> MSVFDRLAGFADSVTNAKQVDVSTATAQKKAEQGVTTPLVSPDAAYQMQAARTGNVGANAFEPGTVQSDFMNLTPMQIMNKYGVEQGLQLINARADAGNQVFNDSVTTRTPGEELGDIATGVGLGFVNTLGGIGALGAGLLNDDAGAVVAQQLSKFNDAVHATQSQALQDKRKLFAARNLMNEVESERQYQTDKKEGTNDIVASLSKFGRDFVGSIENAAQTDSIISDGLAEGVGSLLGAGPVLRGASLLGKAVVPANTLRSAALAGAIDAGTGTQSLARIASTVGRAAPGMVGVGAMEAGGAYQQTADEIMKMSLKDLEKSPVYQQHIKDGMSPEQARRQTASETGLTAAAIQLPIAAATGPLVSRFEMAPFRAGSLGAVGMNLARETVEEGVQGATGQLAQNIAQQQNIDKNQDLLKGVGTQAGLGALYGFGSAGVVQAPAGAARLAGAATAPVLRTTMAGVKAAGSVAGKVVSPIKNTLVARGERVMKQNEEASPVADDYVAQAAQEAMAQAPEAEVTIRDAVEATDATPEQKVAAHQYVSDLMNATRFNPENYQEAPEHIRNAVAGSTDQVQVIQKLADLVNTLDESNPQALMEAASYMYDAVSEFEQFINRDPAALDSIPKDSPAIELLNRYTNLTANIQNTPKVIGALNVINRMINESAQNGSLNVTEESSPQEMQNVALAAEVAPEKLNPESVNVVLKHAADGRIKLNNRQIAALQNAAAILKGAREYDAEAARLGLRPQDIVSKQIKTDESRTQEGQYSALQHANRIRSAYNSGNFELASAYLNDFMQFAQHMQNKVGALNEHLVTGNADKNKSVHYQALTADREWVRSRTGLGVNPYDTKSVKFAQQVALEAKTVADIANALASAYPELKVSHIKVTPLDSRLNAPAAEVVKAFRQGNRDVASSQPKADSVNQVKETPVTKQEPVTSTVQTKTPVSESVKTEPTTKESSPQAIKEPVNQSEKQDVNLTNEDNIKQPTESVKETETSTKESTVTEELKEGIDAVYPSLVGTADSKAEGIKNYFKLSFTLPEEQKSRTVGSEAPLKDVAQALSSRARYELFTEKETANPAFNGEVIKRYKELMEHGEGIADILRSRLAKFLNTKDVGKRFAQGTEANRWVGGKLLNIVEQDGDTFKYNEQLLQTAVLAGLQWRLTATSNTAIKDAKDVAAITGIDQALLPEGLVEQFDTGMTLTEAVSSLAQKIESYWGLSRNPNAPLGYTKGIPTAMAAEILAAFVESTDVVENIVDMSEIDPDNKKTIGLYTIT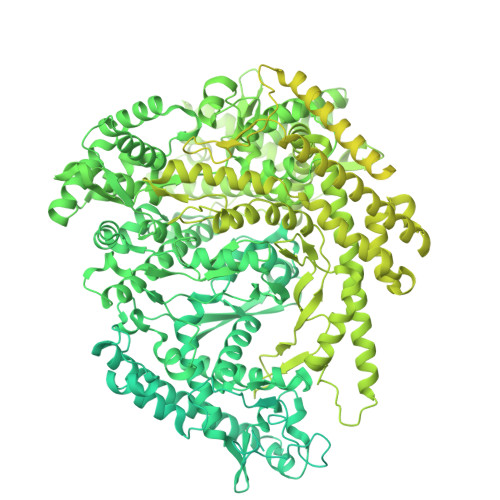ELDSFDPINSFPTAIEEAVLVNPTEKMFFGDDIPPVANTQLRNPAVRNTPEQKAALKAEQATEFYVHTPMVQFYETLGKDRILELMGAGTLNKELLNDNHAKSLEGKNRSVEDSYNQLFSVIEQVRAQSEDISTVPIHYAYNMTRVGRMQMLGKYNPQSAKLVREAILPTKATLDLSNQNNEDFSAFQLGLAQALDIKVHTMTREVMSDELTKLLEGNLKPAIDMMVEFNTTGSLPENAVDVLNTALGDRKSFVALMALMEYSRYLVAEDKSAFVTPLYVEADGVTNGPINAMMLMTGGLFTPDWIRNIAKGGLFIGSPNKTMNEHRSTADNNDLYQASTNALMESLGKLRSNYASNMPIQSQIDSLLSLMDLFLPDINLGENGALELKRGIAKNPLTITIYGSGARGIAGKLVSSVTDAIYERMSDVLKARAKDPNISAAMAMFGKQAASEAHAEELLARFLKDMETLTSTVPVKRKGVLELQSTGTGAKGKINPKTYTIKGEQLKALQENMLHFFVEPLRNGITQTVGESLVYSTEQLQKATQIQSVVLEDMFKQRVQEKLAEKAKDPTWKKGDFLTQKELNDIQASLNNLAPMIETGSQTFYIAGSENAEVANQVLATNLDDRMRVPMSIYAPAQAGVAGIPFMTIGTGDGMMMQTLSTMKGAPKNTLKIFDGMNIGLNDITDASRKANEAVYTSWQGNPIKNVYESYAKFMKNVDFSKLSPEALEAIGKSALEYDQRENATVDDIANAASLIERNLRNIALGVDIRHKVLDKVNLSIDQMAAVGAPYQNNGKIDLSNMTPEQQADELNKLFREELEARKQKVAKARAEVKEETVSEKEPVNPDFGMVGREHKASGVRILSATAIRNLAKISNLPSTQAATLAEIQKSLAAKDYKIIYGTPTQVAEYARQKNVTELTSQEMEEAQAGNIYGWTNFDDKTIYLVSPSMETLIHELVHASTFEEVYSFYQGNEVSPTSKQAIENLEGLMEQFRSLDISKDSPEMREAYADAIATIEGHLSNGFVDPAISKAAALNEFMAWGLANRALAAKQKRTSSLVQMVKDVYQAIKKLIWGRKQAPALGEDMFSNLLFNSAILMRSQPTTQAVAKDGTLFHSKAYGNNERLSQLNQTFDKLVTDYLRTDPVTEVERRGNVANALMSATRLVRDVQSHGFNMTAQEQSVFQMVTAALATEAAIDPHAMARAQELYTHVMKHLTVEHFMADPDSTNPADRYYAQQKYDTISGANLVEVDAKGRTSLLPTFLGLAMVNEELRSIIKEMPVPKADKKLGNDIDTLLTNAGTQVMESLNRRMAGDQKATNVQDSIDALSETIMAAALKRESFYDAVATPTGNFIDRANQYVTDSIERLSETVIEKADKVIANPSNIAAKGVAHLAKLTAAIASEKQGEIVAQGVMTAMNQGKVWQPFHDLVNDIVGRTKTNANVYDLIKLVKSQISQDRQQFREHLPTVIAGKFSRKLTDTEWSAMHTGLGKTDLAVLRETMSMAEIRDLLSSSKKVKDEISTLEKEIQNQAGRNWNLVQKKSKQLAQYMIMGEVGNNLLRNAHAISRLLGERITNGPVADVAAIDKLITLYSLELMNKSDRDLLSELAQSEVEGMEFSIAYMVGQRTEEMRKAKGDNRTLLNHFKGYIPVENQQGVNLIIADDKEFAKLNSQSFTRIGTYQGSTGFRTGSKGYYFSPVAARAPYSQGILQNVRNTAGGVDIGTGFTLGTMVAGRITDKPTVERITKALAKGERGREPLMPIYNSKGQVVAYEQSVDPNMLKHLNQDNHFAKMVGVWRGRQVEEAKAQRFNDILIEQLHAMYEKDIKDSSANKSQYVNLLGKIDDPVLADAINLMNIETRHKAEELFGKDELWVRRDMLNDALGYRAASIGDVWTGNSRWSPSTLDTVKKMFLGAFGNKAYHVVMNAENTIQNLVKDAKTVIVVKSVVVPAVNFLANIYQMIGRGVPVKDIAVNIPRKTSEINQYIKSRLRQIDAEAELRAAEGNPNLVRKLKTEIQSITDSHRRMSIWPLIEAGEFSSIADAGISRDDLLVAEGKIHEYMEKLANKLPEKVRNAGRYALIAKDTALFQGIQKTVEYSDFIAKAIIYDDLVKRKKKSSSEALGQVTEEFINYDRLPGRFRGYMESMGLMWFYNFKIRSIKVAMSMIRNNPVHSLIATVVPAPTMFGNVGLPIQDNMLTMLAEGRLDYSLGFGQGLRAPTLNPWFNLTH> GS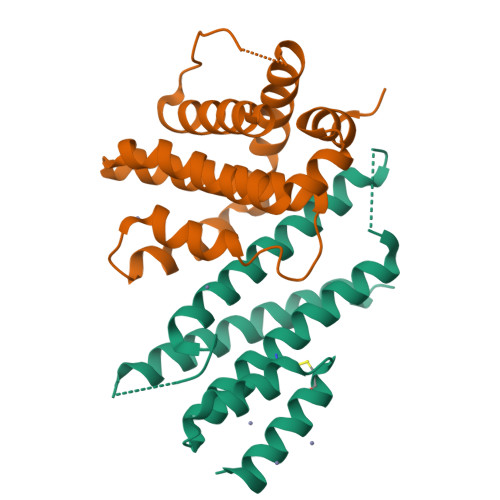HMSTEQIQKRTAAIQKRIAAIQKRIYAMTASGGAGAAGAGAGMSIEEITKQIAAIQLRIVGDQVQIAYQTASGAGAGAGGMSTEEIQKQIAAIETQICKIEAAIELKEAGITSDFYFELINKAKTCEGVEALKEHILAAHT;> GSHMGSDELYRQSLEIISRYLREQATGAKDTKPMGRSGATSRKALETLRRVGDGVQRNHETAFQGMLRKLDIKNEDDVKSLSRVMIHVFSDGVTNWGRIVTLISFGAFVAKHLKTINQESCIEPLAESITDVLVRTKRDWLVKQRGWDGFVEFFHVEDLEGG>MNTPEHMTAVVQR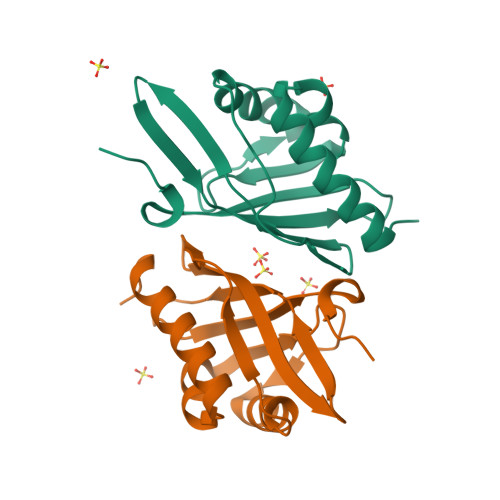YVAALNAGDLDGIVALFADDATVEDPVGSEPRSGTAAIREFYANSLKLPLAVELTQEVRAVANEAAFAFTVSFEYQGRKTVVAPINHFRFNGAGKVVSMRALFGEKNIHAGA[2x]> SGDMADAFGDELFSVFEGDSTTAAGTKKDKEKDKGKWKGPPGSADKAGKRFDGKLQSESTNNGKNKRDVDFEGTDEPIFGKKPRIEESITEDLSLADLMPRVKVQSVETVEGCTHEVALPAEEDYLPLKPRVGKAAKEYPFILDAFQREAIQCVDNNQSVLVSAHTSAGKTVCAEYAIALALREKQRVIFTSPIKALSNQKYREMYEEFQDVGLMTGDVTINPTASCLVMTTEILRSMLYRGSEVMREVAWVIFDEIHYMRDSERGVVWEETIILLPDNVHYVFLSATIPNARQFAEWICHLHKQPCHVIYTDYRPTPLQHYIFPAGGDGLHLVVDENGDFREDNFNTAMQVLRDAGDLAKGDQKGRKGGTKGPSNVFKIVKMIMERNFQPVIIFSFSKKDCEAYALQMTKLDFNTDEEKKMVEEVFSNAIDCLSDEDKKLPQVEHVLPLLKRGIGIHHGGLLPILKETIEILFSEGLIKALFATETFAMGINMPARTVLFTNARKFDGKDFRWISSGEYIQMSGRAGRRGMDDRGIVILMVDEKMSPTIGKQLLKGSADPLNSAFHLTYNMVLNLLRVEEINPEYMLEKSFYQFQHYRAIPGVVEKVKNSEEQYNKIVIPNEESVVIYYKIRQQLAKLGKEIEEYIHKPKYCLPFLQPGRLVKVKNEGDDFGWGVVVNFSKKSNVKPNSGELDPLYVVEVLLRCSKESLKNSATEAAKPAKPDEKGEMQVVPVLVHLLSAISSVRLYIPKDLRPVDNRQSVLKSIQEVQKRFPDGIPLLDPIDDMGIQDQGLKKVIQKVEAFEHRMYSHPLHNDPNLETVYTLCEKKAQIAIDIKSAKRELKKARTVLQMDELKCRKRVLRRLGFATSSDVIEMKGRVACEISSADELLLTEMMFNGLFNDLSAEQATALLSCFVFQENSSEMPKLTEQLAGPLRQMQECAKRIAKVSAEAKLEIDEETYLSSFKPHLMDVVYTWATGA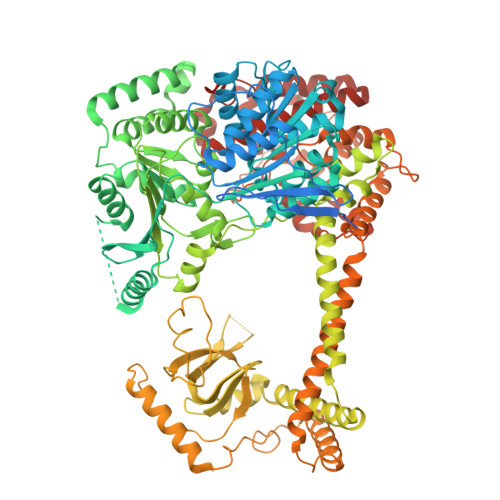TFAHICKMTDVFEGSIIRCMRRLEELLRQMCQAAKAIGNTELENKFAEGITKIKRDIVFAASLYL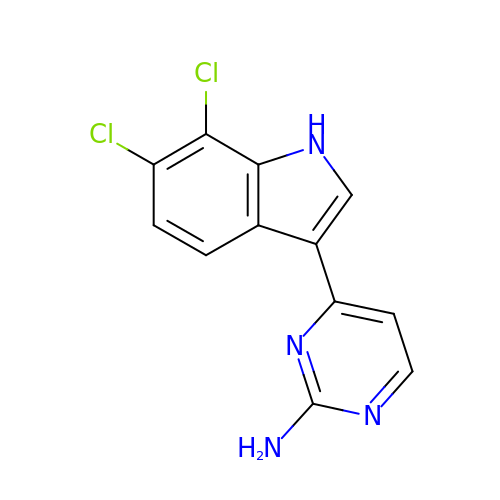4-[6,7-bis(chloranyl)-1~{H}-indol-3-yl]pyrimidin-2-amine | C12 H8 Cl2 N4 | QTGPPZWMCRJECL-UHFFFAOYSA-N1-(5-chloro-2-methylphenyl)-4-(pyrrolo[2,1-f][1,2,4]triazin-4-yl)-1H-pyrrole-2-carboxamide | C18 H14 Cl N5 O | 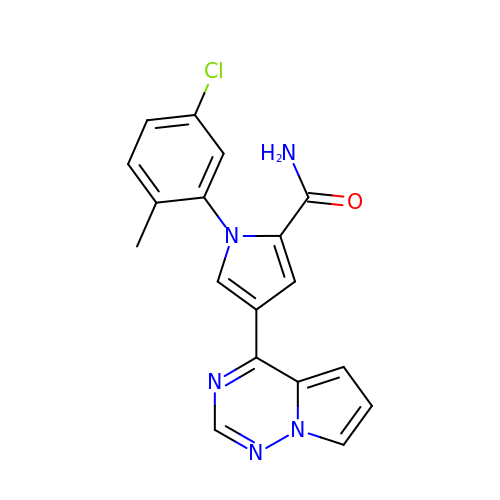LCPNDRXSKAUPSE-UHFFFAOYSA-N>MVLYFIGLGLYDERDITVKGLEIAKKCDYVFAEFYTSLMAGTTLGRIQKLIGKEIRVLSREDVELNFENIVMPLAKENDVAFLTPGDPLVATTHAELRIRAKRAGVESYVIHAPSIYSAVGITGLHIYKFGKSATVAYPEGNWFPTSYYDVIKENAERGLHTLLFLDIKAEKRMYMTANEAMELLLKVEDMKKGGVFTDDTLVVVLARAGSLNPTIRAGYVKDLIREDFGDPPHILIVPGKLHIVEAEYLVEIAGAPREILRVNV[2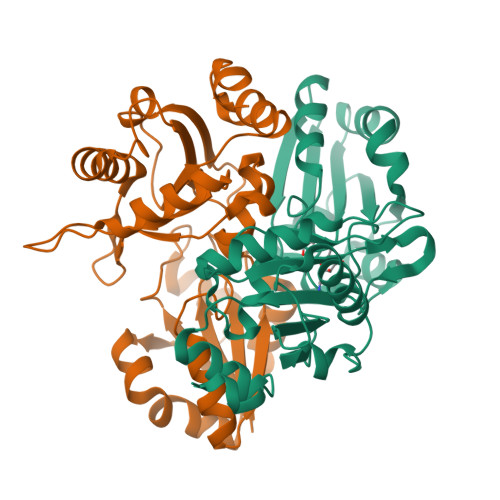x]> MHHHHHHARATGKTF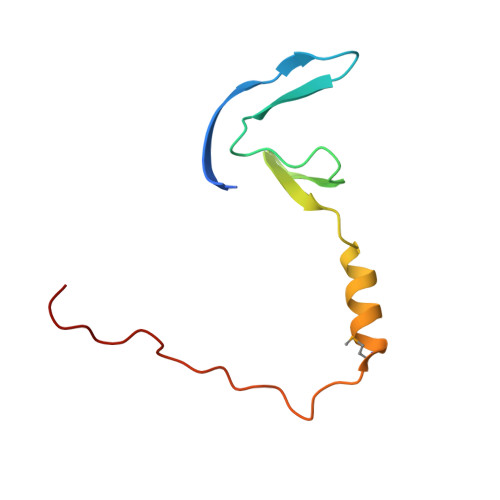RSGNSEAVRLPRDLAFGADVELTLIRSGDVLTIYPSKGSIADLVATLNQMPRPDSVEIRDEDLFPERPGL>[2x]MAHHHHHHVGTNTGGVLVI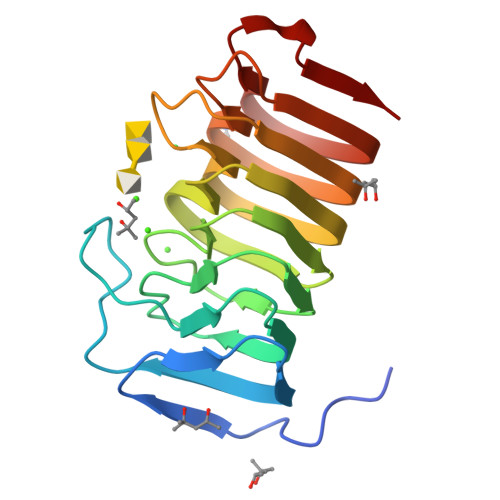TDTIIVKSGQTYDGKGIKIIAQGMGDGSQSENQKPIFKLEKGANLKNVIIGAPGCDGIHCYGDNVVENVVWEDVGEDALTVKSEGVVEVIGGSAKEAANAVFQLNAPCTFKVKNFTATNIGKLVRQNGNTTFKVVIYLEDVTLNNVKSCVAKSDSPVSELWYHNLNVNNCKTLFEFPSQSQIHQY Here, we present the near-atomic resolution structure of Haloferax tailed virus 1 (HFTV1), an archaeal virus thriving in extreme salinity. Through single-particle analysis, we obtained near-atomic resolution maps of DNA-filled and empty virions, enabling us to assemble full atomic models of the virus pre- and post-DNA release, including all structural protein components. The full atomic structure revealed that the virus has a length of 1350 Å and an icosahedral head with a diameter of ~600 Å. The tail has a length of 560 Å and terminates into a baseplate with three radiating TFs of ~190 Å in length.

The BPH also anchors three TFs. The TFs are formed as a homotrimer of gp42 [TF protein (TFP)]. Three TFPs come together to form a base, followed by a β-helix, a stalk, and a head. The TFs are connected to the N terminus of each BPH subunit and radiate away at a ~45°. This interaction is stabilized by extensive hydrogen bonds and Mg2+ ion coordination. A DynaMight analysis revealed that the TFs are highly flexible with respect to the BPH, likely aiding their ability to dock to the S-layer at the cell surface.

> MPQLGDSKLGESQLGSPGTLKQGVEWTVVVDGEEQNNVWDVQVVDTANPFGDYAVFKMDDRGGQAFEAYPRGTRVEAYVSEGTEPLDNRFTGYVVERRENEQQGADVLEVEAYSFDQFLRRNTVTNDQTGNTISQALADIIQTDTPVRFNAANITVGDDQELTRSYQGDPVENALRDFAFKSTNEDFGVGDDLEFFFQPRETVHIDRGVDNTQWFRYDIPELGKEAINEVEVWFDDGEESVIVDDGTDKLDLQDSLGLPSPGTQRKELQRPLVTDISDAEDIGRKYLAFRNSTLSGTVTTYGLYDAEPGDTIDITIDPRGIDEEFVIAAIEYRWGVDETILTVVEKRGDVDDILSELSESVQRIEMQGANRDAPKNRITTTNAAAIVSVDVDAGGTSADADRFVNDGRNAVRDAWTGAGNPDIANIVVGDDNSGLSRTNTTLGNQTDSVSVTESLPSAKVVEYSATLTQSGVEEIGLETSTGTLLTRATFETPVDLSSDTVTVTLTVSNDDSVSRGVMTNDGQTAVRDVLADNSPTLPTDYGYGDDSTAVAETDTTLGNELANTSLEEILIQSASSVSAWNTILGTLASTYPLVVSSSGIRPAQTAWTTESDNLAQSGTALVTVGDYSNGEAEGLDSPGDTLELSFTPEHDIPGEEFALWCRIETDLGGTDPGPEITVTLDIDGDTYSWVPIGTNTALGLNWYDLANNTFGGSSTYPDTDIPEGSTVTLSIEATSSSVSGQGHAVDVMAPLDALTRVTGGSDATSAYTFDNNNGGSGGYLDGPELYPDQLILSLETATTRRNVSEARFTLTANDTSGNFYVELANDGSTFNRVNNATSGSVTFASPDTNVDTNISLNRYGSRSTATPQTGFNAQEIDNWELYADIDAVLPDDIGVTLSRAIIPPNTSGIVGQTVREAGLKSGSTLLTRHILAEFLLDTDQRLASSESTRFTSDN;>[3x]MADTTIIDAVVFPQDDGTGVSNGDEDYDSAGYLASLARYAGDGSYVGGDSTGSPTLQFANIDTANEEVDIQPGHAFILESGHIVQSGSQKTYDTNLPDSVPYVVILPSSVTNVPLDTDVDNDVWLAVDPTSNDSVYIRSGNGLSAPSDPSVKLGTVNSSTGSTTRPNDLADHSVDALNATTIDASDTVTGDTVDATTTLTDAAGVSHTGELEDINHGSKHEDGGSDEISVGGLSGDLADPQDPKAHAASHSADSADEISVENLSTTGSADTVPISQGDGTLSMGSIVPTDLQWREDSNSPQTDTNVGTSTYTIADTFDEYLIRVQVFEESSAPGTVELRAEGNSQSSYDYISEDGTTTSAATSIPCIELQADSSTISVFGASGRFSGQWEFRSQPNTSTNLATAGFLAVISSPLGSLELFRAANNFSVTWEVFGRDIGPAGVP6-methyl-3,9-dihydro-2H-purin-2-one | C6 H6 N4 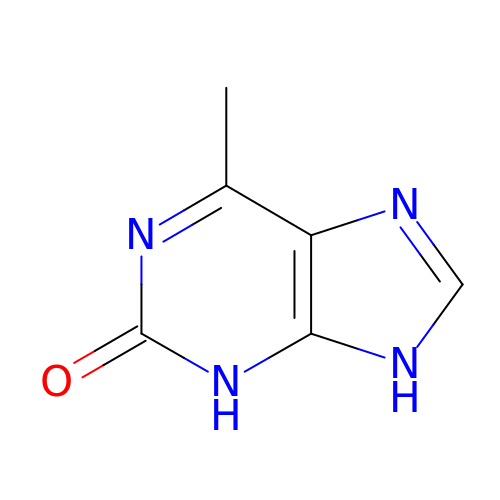O | PTQIZCPBAIYYII-UHFFFAOYSA-N4-(2-chloroethyl)benzoic acid | C9 H9 Cl O2 | 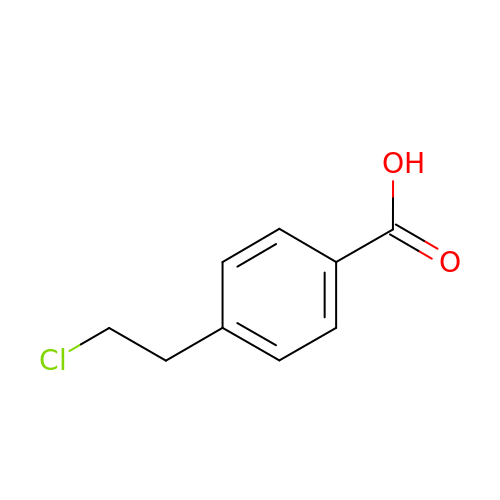OOAPBGPLZAFZSO-UHFFFAOYSA-N>[2x]MVCGREGEEKPPLSAETQWKDRAETVIIGGGC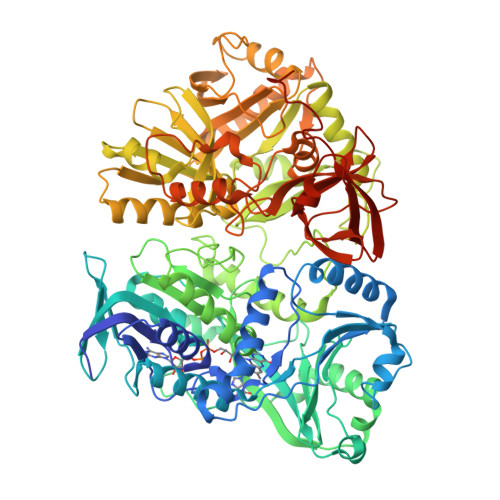VGVSLAYHLAKAGMKDVVLLEKSELTAGSTWHAAGLTTYFHPGINLKKIHYDSIKLYEKLEEETGQVVGFHQPGSIRLATTPVRVDEFKYQMTRTGWHATEQYLIEPEKIQEMFPLLNMNKVLAGLYNPGDGHIDPYSLTMALAAGARKCGALLKYPAPVTSLKARSDGTWDVETPQGSMRANRIVNAAGFWAREVGKMIGLEHPLIPVQHQYVVTSTIPEVKALKRELPVLRDLEGSYYLRQERDGLLFGPYESQEKMKVQDSWVTNGVPPGFGKELFESDLDRIMEHIKAAMEMVPVLKKADIINVVNGPITYSPDILPMVGPHQGVRNYWVAIGFGYGIIHAGGVGKYLSDWILHGEPPFDLIELDPNRYGKWTTTQYTEAKARESYGFNNIVGYPKEERFAGRPTQRVSGLYQRLESKCSMGFHAGWEQPHWFYKPGQDTQYRPSFRRTNWFEPVGSEYKQVMQRVAVTDLSPFGKFNIKGQDSIRLLDHLFANVIPKVGFTNISHMLTPKGRVYAELTVSHQSPGEFLLITGSGSELHDLRWIEEEAVKGGYDVEIKNITDELGVLGVAGPQARKVLQKLTSEDLSDDVFKFLQTKSLKVSNIPVTAIRISYTGELGWELYHRREDSVALYDAIMNAGQEEGIDNFGTYAMNALRLEKAFRAWGLEMNCDTNPLEAGLEYFVKLNKPADFIGKQALKQIKAKGLKRRLVCLTLATDDVDPEGNESIWYNGKVVGNTTSGSYSYSIQKSLAFAYVPVQLSEVGQQVEVELLGKNYPAVIIQEPLVLTEPTRNRLQKKGGKDKTRP>[4x]MRVLIIGAGILGASAAYHLARLGAQVEIIDQNHPGKATLAGAGVVCPWATEADDPDWYLLYARGARYYGTLIEELRGQGETELGYSRVGALVLAEDRARLDTIEGRISR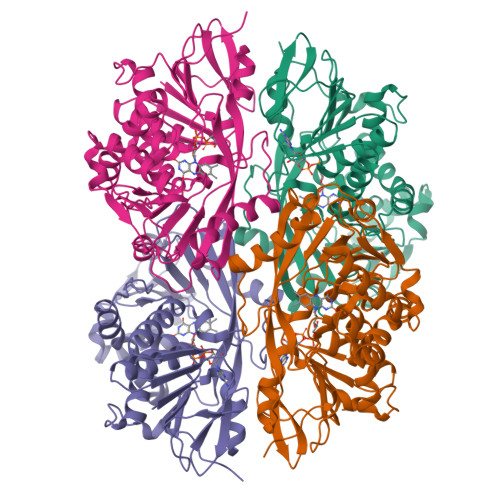RIKDAPEAGTVRRLGAGEAKRLFPPLRDDLEAIHIPGGARVDGRLLAASMLRVAISSGATLRNDYVSLRLNDGRAECLGSDGRPIPADEIIVTAGAWAAQILALLGLRHPVVPQKGQIIHLHLPGVATSGWPVVLPMNSYYMLAFDDSRVVVGATREDGSGFDYRVTARGQLEVLQAGLGIAPGLADATHIETRVGFRPAGSAMRPILGRVPQIAGLTIGNGLGASGLTVGPFAGHLLAGVVMGEPAEVPLERYSPTGPEAGLEHHHHHH(2R)-2-(4-hydroxy-3-methoxyphenyl)-3-(pyridin-2-ylmethyl)-1,3-thiazolidin-4-one | C16 H16 N2 O3 S | 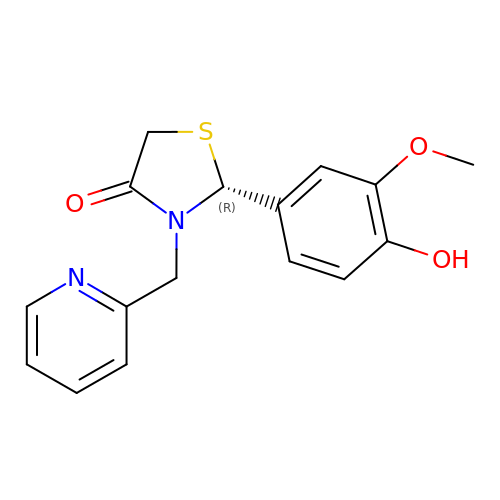HHJAKBZAUFYRBJ-MRXNPFEDSA-N> GSMVEATAQETDRPRFSFSIAAREGKARTGTIEMKRGVIRTPAFMPVGTAATVKALKPETVRATGADIILGNTYHLMLRPGAERIAKLGGLHSCMGWDRPILTDSGGYQVMSLSSLTKQSEEGVTFKSHLDGSRHMLSPERSIEIQHLLGSDIVMAFDESTPYPATPSRAASSMERSMRWAKRSRDAFDSRKEQAENAALFGIQQGSVFENLRQQSADALAEIGFDGYAVGGLAVGEGQDEMFRVLDFSVPMLPDDKPHYLMGVGKPD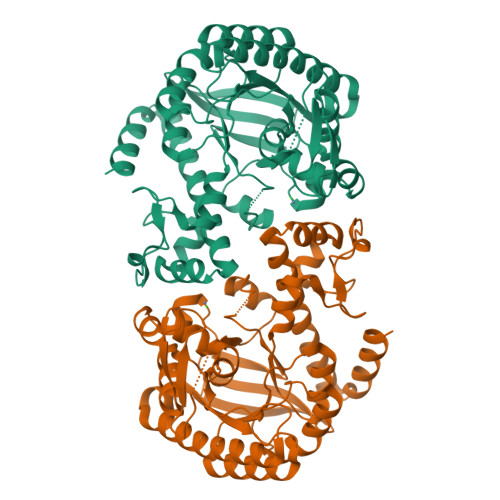DIVGAVERGIDMFDSVLPTRSGRNGQAFTWDGPINIRNARFSEDLKPLDSECHCAVCQKWSRAYIHHLIRAGEILGAMLMTEHNIAFYQQLMQKIRDSISEGRFSQFAQDFRARYFARNS> SGHSSVVVDTNGQPVSNGADAYYLVPVSHGHAGLALAKIGNEAEPRAVVLDPHHRPGLPVRFESPLRINIIKESYFLNIKFGPSSSDSGVWDVIQQDPIGLAVKVTDTKSLLGPFKVEKEGEGYKIVY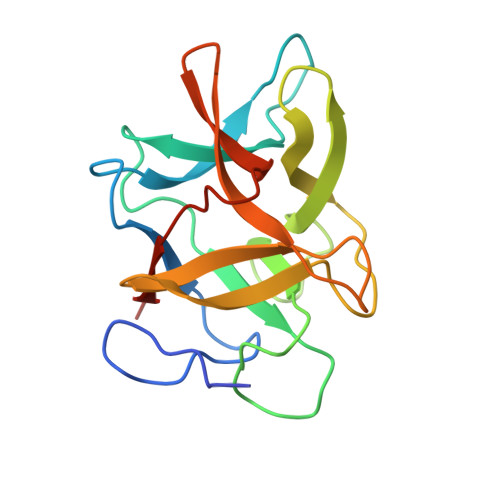YPERGQTGLDIGLVHRNDKYYLAVKDGEPCVFKIRKATDE> KELNDLEKKYNAHIGVYALDTKSGKEVKFNSDKRFAYASTSKAINSAILLEQVPYNKLNKKVHINKDDIVAYSPILEKYVGKDITLKALIEASMTYSDNTANNKIIKEIGGIKKVKQRLKELGDKVTNPVRYEIELNYYSPKSKKNTSTPAAFGKTLNKLIANGKLSKENKKFLLDLMLNNKSGDTLIKDGVPKDYKVADK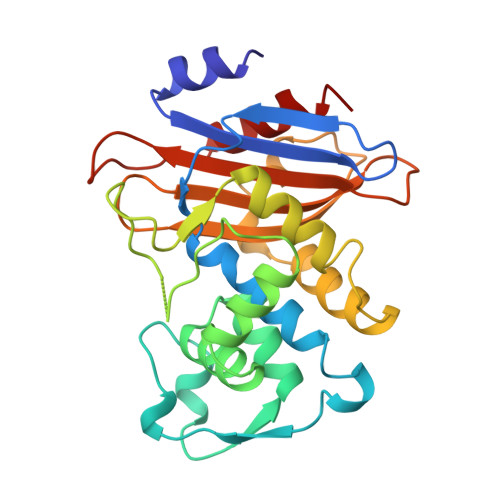SGQAITYASRNDVAFVYPKGQSEPIVLVIFTNKDNKSDKPNDKLISETAKSVMKEF~{N}-[(1-cyclobutyl-1,2,3-triazol-4-yl)methyl]-3-(1~{H}-indazol-3-yl)-5-(propanoylamino)benzamide 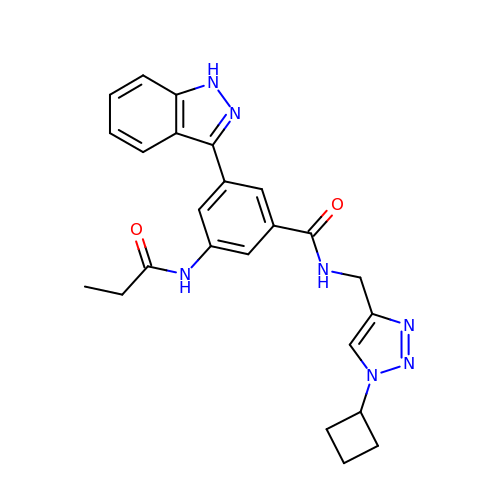| C24 H25 N7 O2 | BPAOQMOHTMHCAO-UHFFFAOYSA-N>[2x]MSRV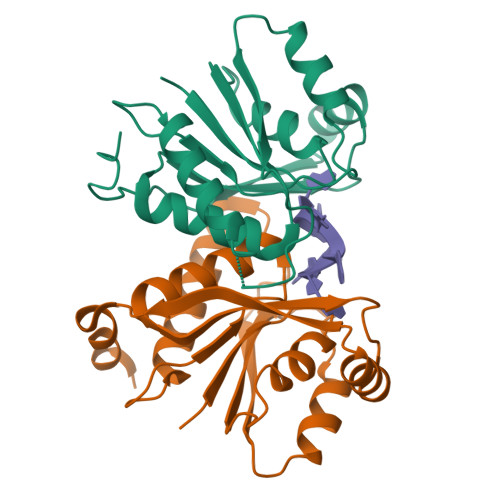LLCSAGHSSMVVPEAFHAVPEGFEEVHVFTTDSEKFNPVVLNDFFHSLPNVRFSITKCHGLADILNERDFEFYQEMLWQWYLTKMPDNELPYVCLSGGIKSMSASLQKAATLFGAQSVFHVLADNNPRNIEEMFDALQKGQIHFIEMGYEPGWAALRRLKKILPINEGCSRDNFKPLISKS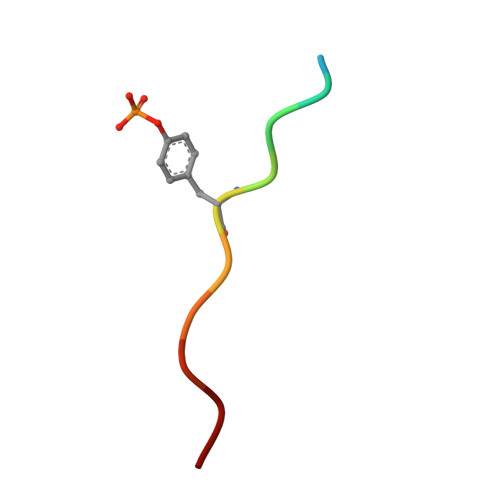> KSLTIYAQVQK N-(5'-PHOSPHOPYRIDOXYL)-D-ALANINE | C11 H17 N2 O7 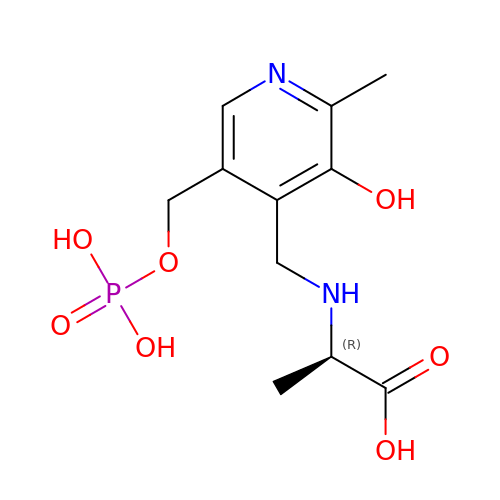P | WACJCHFWJNNBPR-SSDOTTSWSA-N> NYMGNPWTEYMAKYDIEEVHGSGIRVDLGEDAEVAGTQYRLPSGKCPVFGKGIIIENSNTTFLKPVATGNQDLKDGGFAFPPTNPLISPMTLNGMRDFYKNNEYVKNLDELTLCSRHAGNMNPDNDKNS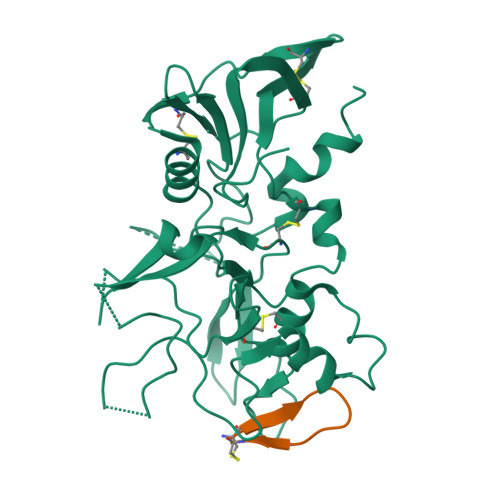NYKYPAVYDYNDKKCHILYIAAQENNGPRYCNKDQSKRNSMFCFRPAKDKLFENYTYLSKNVVDNWEEVCPRKNLENAKFGLWVDGNCEDIPHVNEFSANDLFECNKLVFELSASDQPKQYEQHLTDYEKIKEGFKNKNASMIKSAFLPTGAFKADRYKSHGKGYNWGNYNRETQKCEIFNVKPTCLINNSSYIATTALSHPIEVE;> CWTTRMSPPQQIC>AIADVGTDRYAPYFAYAAAQPSDEVTTVRGLSNPLIKTAPVTLPFDLGQAVADNCLSLSGMGYYLGLGGCCPTCAAAEPRLGRSDRAALVLAYVQQLNSIYEYRVFLASVAARDPSERALEEVLAHPELFFAYYVLRDGGLRDVRVLFFEDPDAQGALMMYVVFPEKSVHVHHRVLDRLLGACAGHRIVAHVWQTMFVLVVRKKGDGRPADDVPAVSASDIYCKMRDISFDGELLLEYKRLYAAFEDFRPPRP[42x];>MSGTLVQRLKLILSGGNLRCSDGETACDPERPPTRCVFQVHGQDGSNDTFPL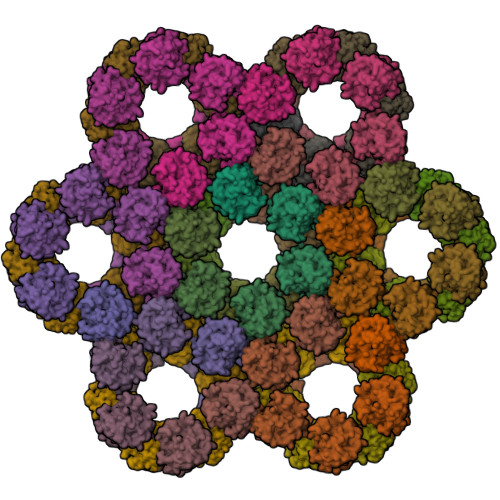EYVLRLMRSWAHVPCDPYVRVQNTGVSVLFQGFFFRPADAPLAAITAEHNNVILASTHSTGMSLSALDDIKRAGGVDTRPLRAMMSVSCFVRMPRVQLSFRFMGPDDASQTQRLLDRAEMRQRSVSR[42x]> GSMRETAIQQLEADILDVNQIFKDLAMMIHDQGDLIDSIEANVESSEVHVERASDQLQRAAYYQKKSRK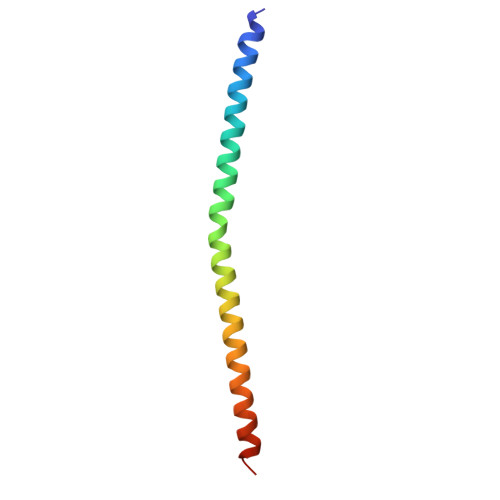KM>[2x]M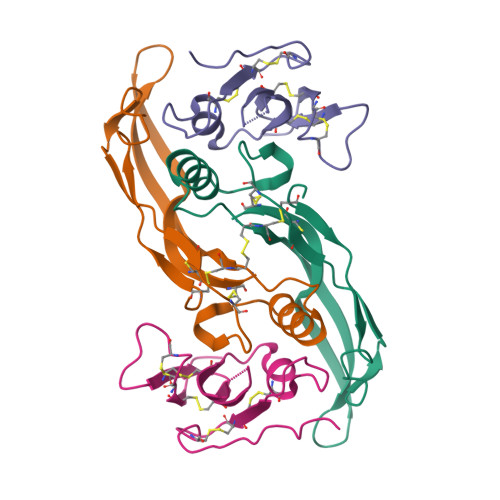AQAKHKQRKRLKSSCKRHPLYVDFSDVGWNDWIVAPPGYHAFYCHGECPFPLADHLNSTNHAIVQTLVNSVNSKIPKACCVPTELSAISMLYLDENEKVVLKNYQDMVVEGCGCR;>TLPFLKCYCSGHCPDDAINNTCITNGHCFAIIEEDDQGETTLASGCMKYEGSDFQCKDSPKAQLRRTIECCRTNLCNQYLQPTLPPVVI[2x]>SGRGEAETRECIYYNANWELERTNQSGLERCEGEQDKRLHCYASWR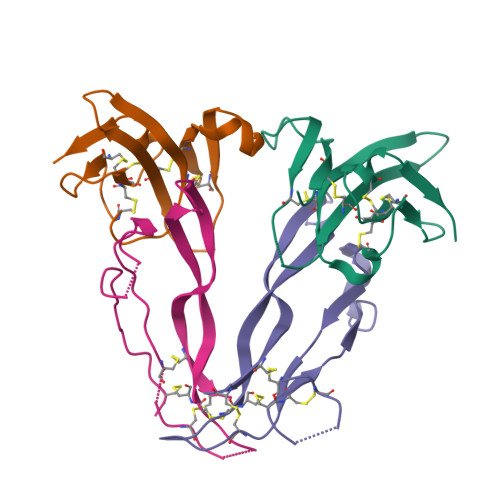NSSGTIELVKKGCWLDDFNCYDRQECVATEENPQVYFCCCEGNFCNERFTHLPEPLVPR[2x];>GLECDGKVNICCKKQFFVSFKDIGWNDWIIAPSGYHANYCEGECPSHIAGTSGSSLSFHSTVINHYRMRGHSPFANLKSCCVPTKLRPMSMLYYDDGQNIIKKDIQNMIVEECGCS[2x]One such system is the PreQ1 riboswitch, which binds to the small, modified nucleotide 7-aminomethyl-7-deazaguanine (known as PreQ1). Upon recognition of PreQ1, the RNA changes conformation and alters gene expression at either transcriptional level or translational level. For the PreQ1 riboswitch from Thermoanaerobacter tengcongensis (Tt-preQ1-RS) binding to PreQ1 also results in the formation of an H-type pseudoknot structure. However, in this case the riboswitch acts at the translational level by regulating the accessibility of the Shine-Dalgarno sequence and ribosome binding.

Co-crystals were obtained using wild type (WT) and an abasic mutant at positions 13 and 14 (ab_13-14) without photocrosslinking, and the complex structures were solved by the molecular replacement method at 2.80 and 1.57 Å resolution respectively. In contrast, when using abasic mutant at positions 13 and 14, larger co-crystals were obtained that diffracted to 1.6 Å resolution. Importantly, the binding mode of the compound is conserved between the WT and abasic mutant crystals and the RNA structures are quite similar with the exception of the nucleotides from positions 12 to 14. No specific interaction is observed between the alkyne handle and the RNA, suggesting that positions 12 to 14 are not involved in the direct interaction for binding of the compound 11. Based on these findings, it was concluded that a high-resolution co-crystal structure of the abasic mutant is more informative in terms of evaluating the chemical determinants of this interaction. From inspection of the structure, it is clear that the PreQ1 portion of 11 binds to the Tt-preQ1-RS aptamer in an analogous mode to the native ligand, making near identical contacts. The methylamine group hydrogen-bonds with O6 of G5. However, the hydrogen bond between N7 of G5 and the methylamine group was not observed in the present crystal structure. This is likely due to the impact of the extended linker on N7, which is flexible and may interfere with this interaction. The sidechain of the probe projects out of the binding pocket toward the solvent and is proximal to two guanosines (G4 and G5) that it could potentially modify upon irradiation. Thus, it is clear that modification of the exocyclic amine of PreQ1 does not dramatically alter its mode of binding to RNA, though it does decrease affinity.

> CUGGGUCGCAGUNNCCCCAGUUAACAAAACAAG>SNAKQTWHANFLVIDKMGVLITGEANIGKSELSLALIDRGHQLVCDDVIDLKQENNQLIGSCPSVANGYILITGIGI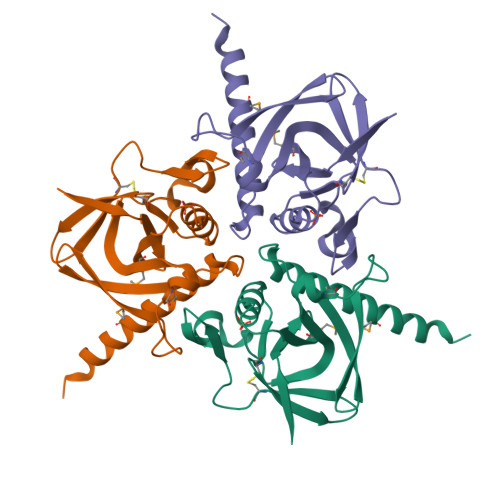IDVPKLFGLDAVVNQHEVHLSISLVKPEKMPLLDDPLNPLYRTEIILGINVPKILFPIHPGRNLPLLIETLVRNHRLKMEGYDSSHHFHEHFRKARDNYDSKKN[2x]> GSHMASMAKTLKDLQGWEIITTDEQGNIIDGGQKRLRRRGAKTEHYLKRSSDGIKLGRGDSVVMHNEAAGTYSVYMIQELRLNTLNNVVELWALTYLRWFEVNPLAHYRQFNPDANILNRPLNYYNKLFS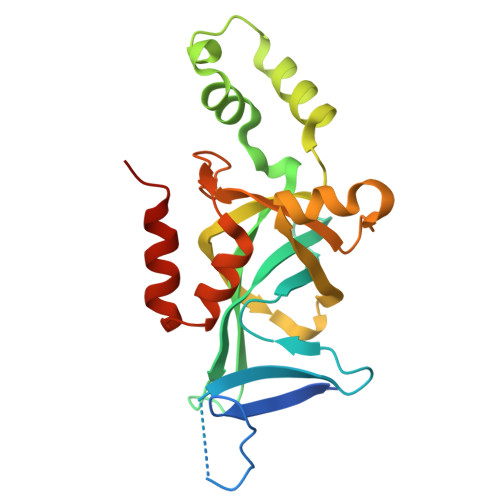ETANKNELYLTAELAELQLFNFIRVANVMDGSKWEVLKGNVDPERDFTVRYICEPTGEKFVDINIEDVKAYIKKVEPREAQEYLKDLTLPSKKKE> FDFNIMVVGQSGLGKSTLVNTLFKSQVSRKASSWNREEKIPKTVEIKAIGHVIEEGGVKMKLTVIDTPGFGDQINNENCWEPIEKYINEQYEKFLKEEVNIARKKRIPDTRVHCCLYFIS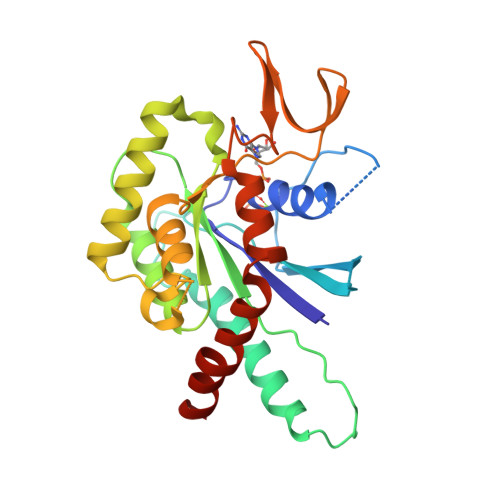PTGHSLRPLDLEFMKHLSKVVNIIPVIAKADTMTLEEKSEFKQRVRKELEVNGIEFYPQKEFDEDLEDKTENDKIRQESMPFAVVGSDKEYQVNGKRVLGRKTPWGIIEVENLNHCEFALLRDFVIRTHLQDLKEVTHNIHYETYRAKRLN> MGHHHHHHSHMRPLTEEETRVMFEKIAKYIGENLQLLVDRPDGTYCFRLHNDRVYYVSEKIMKLAANISGDKLVSLGTCFGKFTKTHKFRLHVTALDYLAPYAKYKVWIKPGAEQS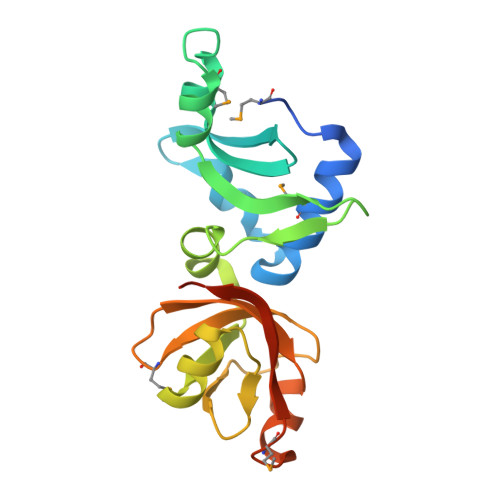FLYGNHVLKSGLGRITENTSQYQGVVVYSMADIPLGFGVAAKSTQDCRKVDPMAIVVFHQADIGEYVRHEETLT> MNYATVNDLCARYTRTRLDILTRPKTADGQPDDAVAEQALADASAFIDGYLAARFVLPLTVVPSLLKRQCCVVAWFYLNESQPTEQITATYRDTVRWLEQVRDGKTDPGVESRTA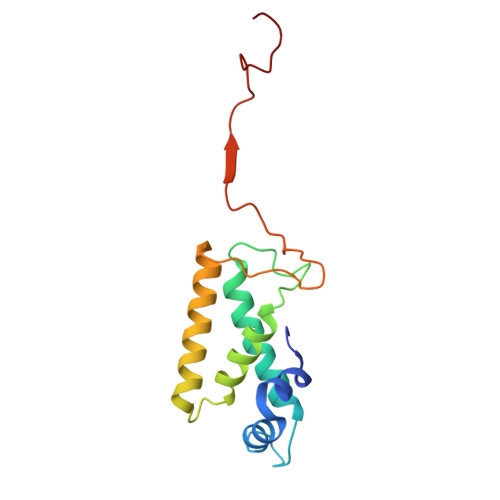ASPEGEDLVQVQSDPPVFSRKQKGFI> DIPQQLVERLQEEKRIEAQKRKERQEAHLYMQVQIVAEDQFCGHQGNDMYDEEKVKYTVFKVLKNSSLAEFVQSLSQTMGFPQDQIRLWPMQARSNGTKRPAMLDNEADGNKTMIELSDNENPWTIFLETVDPELAASGATLPKFDKDHDVMLFLKMYDPKTRSLNYCGHIYTPISCKIRDLLPVMCDRAGFIQDTSLILYEEVKPNLTERIQDYDVSLDKALDELMDGD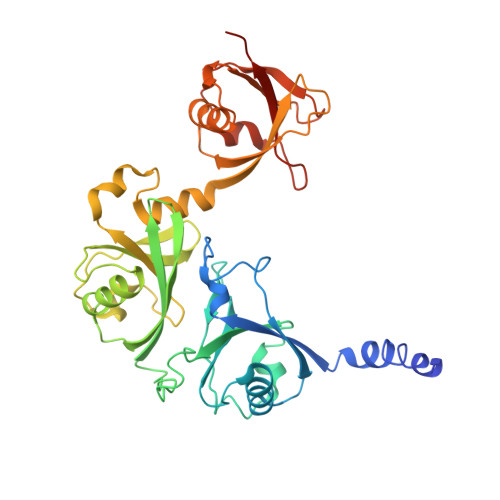IIVFQKDDPENDNSELPTAKEYFRDLYHRVDVIFCDKTIPNDPGFVVTLSNRMNYFQVAKTVAQRLNTDPMLLQFFKSQGYRDGPGNPLRHNYEGTLRDLLQFFKPRQPKKLYYQQLKMKITDFEN> MLLKDRVILITNVEKFAGHGTTRIALAQGATVLAHDPSFDTPSARHKYESQFPGAHALSAVEPAAMVELALKRHGHIDALVNNDAYPALKAPLGEARIEDFRDALEVMAVAPFRLTQLVAPSMRKRKSGRIVFVSSAAPLRGIANYAPYVSARAAGNGLVSS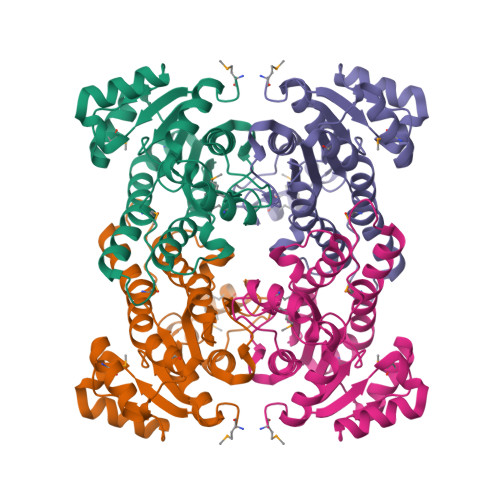LAKELGRDSITVNAVGSNYVENPDYFPPALLANREAMAKMTAQIPLGRLGKSDELGATICFLCSDGAGFITGHVLPHAGGWA> HHHHHHMIVLFVDFDYFYAQVEEVLNPSLKGKPVVVCVFSGRFEDSGAVATANYEARKFGVKAGIPIVEAKKILPNAVYLPMRKEVYQQVSSRIMNLLREYSEKIEIASIDEAYLDISDKVRDYREAYNLGLEIKNKILEKEKITVTVGISKNKVFAKIAADMAKPNGIKVIDDEEVKRLIRELDIADVPGIGNITAEKLKKLGINKLVDTLSIEFDKLKGMIGEAKAKYLISLARDEYNEP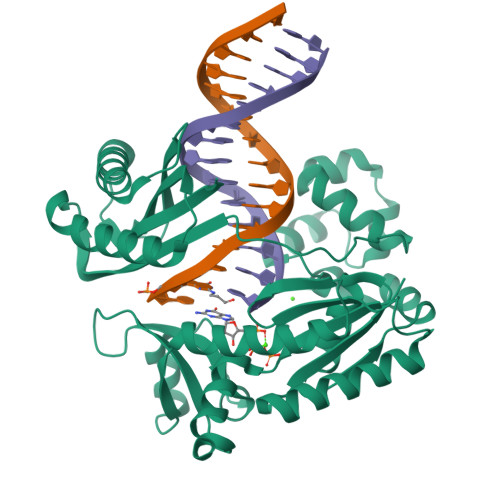IRTRVRKSIGRIVTMKRNSRNLEEIKPYLFRAIEESYYKLDKRIPKAIHVVAVTEDLDIVSRGRTFPHGISKETAYSESVKLLQKILEEDERKIRRIGVRFSKFI> MNYTKFDVKNWVRREHFEFYRHRLPCGFSL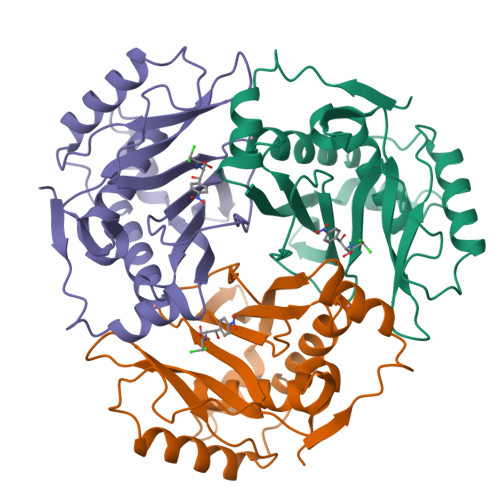TSKIDITTLKKSLDDSAYKFYPVMIYLIAQAVNQFDELRMAIKDDELIVWDSVDPQFTVFHQETETFSALSCPYSSDIDQFMVNYLSVMERYKSDTKLFPQGVTPENHLNISALPWVNFDSFNFNVANFTDYFAPIITMAKYQQEGDRLLLPLSVQVHHAVCDGFHVARFINRLQELCNSKLK Oligopeptidase B (OpB) is a two-domain, trypsin-like serine peptidase belonging to the S9 prolyloligopeptidase (POP) family. Two domains are linked by a hinge region that participates in the transition of the enzyme between two major states—closed and open—in which domains and residues of the catalytic triad are located close to each other and separated, respectively. In this study, we described for the first time the structures of bacterial OpB from S. proteomaculans (PSP) obtained by X-ray for an enzyme with a modified hinge region (PSPmod) and two of its derivatives. The enzymes were crystallized in the presence of spermine and adopted uncommon intermediate states in the crystal lattices.

Despite its small effect on thermal stability, the presence of Sp made it possible to obtain crystals suitable for X-ray analysis for PSPmod and its derivatives, PSPmodE125A and PSPmodS532A. PSPmodS532A carried the alanine substitution of the catalytic triad serine and did not possess any enzymatic activity. PSPmod and two its derivatives (PSPmodE125A and PSPmodS532A) were crystallized in intermediate conformations, which are characterized by a disruption of the catalytic triad typical for ligand-free enzymes in open states, while domains’ closeness resembled closed states of ligand-bound POP. In the PSPmod structure, the distances between Cα-atoms in the pairs Ser532–His652 and His652–Asp617 are equal to 18.2 and 10.6 Å, respectively, which are longer than those in the closed states of TbOpB and ApPEP and comparable with those in the open state of TbOpB and intermediate states of PfPEP and GmPEP. Similar distances are observed in the structures of PSPmod derivatives. As a result, five, three and two bound Sp molecules were found in the structures of PSPmod, PSPmodE125A and PSPmodS532A, respectively. Sp701 is present in all structures, while Sp704—only in the PSPmod structure. The second Sp of the PSPmodS532A structure is in the proximity of catalytic Ser532 similarly to Sp703 in the PSP structure.

> MTPPKAEKRPYPITTHGDTRVDDYYWLRDDERTDPQVLDYLQAENAFTDAALKPQQALRETLYEEMVARENLYFQSVPYVRHGYRYQTRFEPGNEYAIYVRQPQAESEHWDTLIDGNQRAEQREFYTLGGLEVSPDNQKLAVAEDFLSRRQYDIRFKNLSDDSWTDEVLENTSGSFEWANDSATVYYVRKHAKTLLPYQVYRHVVGTDPQLDELIYEEQDDTFYVGLEKTTSDRFILIHLSSTTTSEILLLDADRADSTPQMFVPRRKDHEYGIDHYHQHFYIRSNKDGKNFGLYQSEQADEAQWQTLIAPRIEVMLEGFSLFRDWLVVEERSEGLTQLRQIHWQSGEVKRIAFDDPTYTTWLAYNPEPETELLRYGYSSMTTPTTLYELNLDSDERVMLKQQEVKNFTPENYRSERVWVKARDGVEVPVSLVYRHDSFARGTNPLMVYGYGSYGSSMDPAFSASRLSLLDRGFVFVLAHIRGGGELGQLWYEDGKLFKKQNTFNDFIDVTEALIAQGYGDAKRVFAMGGAAGGLLMGAVINQAPELFNGIVAQVPFVDVVTTMLDESIPLTTGEYDEWGNPNQQAYYDYILQYSPYDQVKAQDYPHMLVTTGLHDSQVQYWEPAKWVAKLRELKTDDRQLLLYTDMDSGHGGKSGRFKAYEDIALEYAFILALAE>[2x]MASSHHHHHHSSGLVPRGSHMNDAAVITGSDTGAVTEDESTPLLTETGTLSVTDVDGADEAKFQAGNGTPSAGALGSLTITEGGAWTYNVDNSKVQYLGEGETKVETFTVASVDGTTHTVTITITGVNDAAVITGSDTGAVTEDESNPTLTE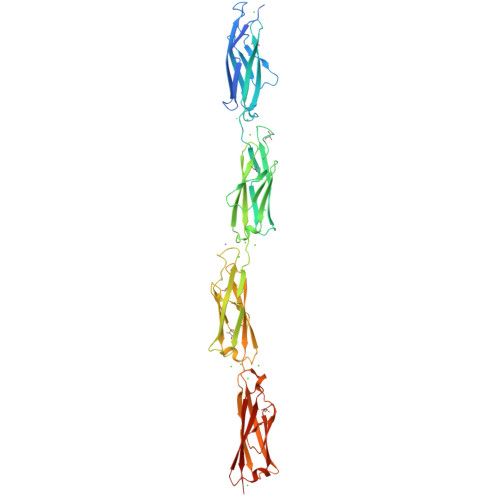TGTLSVTDVDGADEAKFLAGNGTPSAGALGSLTITEGGAWTYNVDNSKVQYLGEGETKVETFTVASVDGTTHTVTITITGVNDAAVISGSDTGAVTEDESTPLLTETGTLSVTDVDGADEAKFLAGNGVASNGALGSLTITEGGAWTYNVDNSKVQYLGEGETKVETFTVASVDGTTHTVTITITGVNDAAVISGSDTGAVTEDETNPLLTETGTLSVTDVDGADEAKFLAGNGTPSAGALGSLTITEGGAWTYNVDNSKVQYLGEGETKVETFTVASVDGTTHTVTITITGVNDGA> GMASLPKRIIKETEKLVSDPVPGITAE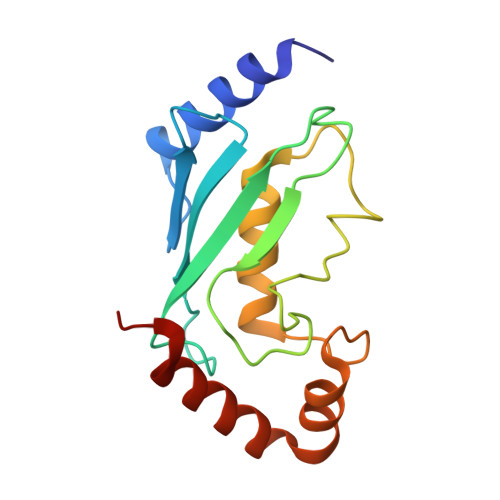PHDDNLRYFQVTIEGPEQSPYEDGIFELELYLPDDYPMEAPKVRFLTKIYHPNIDRLGRICLDVLKTNWSPALQIRTVLLSIQALLASPNPNDPLANDVAEDWIKNEQGAKAKAREWTKLYAKKKPE Encapsulins are a class of BMCs characterised by their conserved subunit (Enc), which self-assembles to encapsulate enzymatically active cargoes and can remain porous to cargo substrates. The overall structure of Enc subunits across species with different T numbers is conserved and consists of a peripheral domain (P-domain), an axial domain (A-domain), and an extension loop (E-loop). T = 1 encapsulins of Mycobacterium tuberculosis, the causative agent of tuberculosis, and the closely related Mycobacterium marinum, are known to encapsulate the DyP as a core cargo with iron storage ferritin protein (BfrB)28 and FolB as possible secondary cargoes. In vitro cryo-electron microscopy (EM) single-particle analysis of the Mycobacterium tuberculosis encapsulin was used to obtain three structures of the encapsulin shell in intermediate states, as well as a 2.3 Å structure of the fully assembled shell.

In addition, we studied partial encapsulin structures to characterise stable encapsulin shell intermediates in vitro, by using low pH conditions to disassemble encapsulin shells, followed by reassembly at neutral pH. To explore the structural landscape of encapsulin shell formation, we used 2D and 3D (focused) classification and local symmetry to determine the structure of different stable encapsulin intermediates in an incomplete assembly state. This resulted in structures of three distinct intermediates of the encapsulin shell; a 48-mer (3,427 particles, 5.4 Å), a 52-mer (4,378 particles, 4.5 Å) and a 54-mer (6,294 particles, 4.6 Å). All three intermediates have an even number of monomers, appear to be closed on one side of the shell, and miss subunits on the other end. All three stable intermediates have an overall icosahedral structure with RMSD values for the 48,52 and 54-mer compared to the structure of the full shell of 1.08 Å, 0.60 Å and 2.66 Å respectively, although the 54-mer is, compared to the full encapsulin, flattened in one direction and elongated perpendicularly to it. The 52-mer consists of 39 fully resolved, and 13 less well resolved monomers, and the 54-mer consists of 27 fully resolved monomers and 27 less well resolved monomers. Not surprisingly, we observed higher cross-correlation values for Enctb monomers on the far side of the opening and lower cross-correlation values closer to the opening; in particular directly on the edges. On the edges of the intermediate encapsulin shells, we observed many points of three and fivefold symmetry with one or more Enctb subunits missing. However, all dimers (in total 77) have both Enctb subunits present, and where a subunit around five or three fold symmetry is missing, its dimeric partner is also missing. Our intermediate structures indicate that the structure of larger partial shells is largely icosahedral, with some deviations observed in the 54-mer.

>[54x]MNNLYRDLAPVTEAAWAEIELEAARTFKRHIAGRRVVDVSDPGGPVTAAVSTGRLIDVKAPTNGVIAHLRASKPLVRLRVPFTLSRNEIDDVERGSKDSDWEPVKEAAKKLAFVEDRTIFEGYSAASIEGIRSASSNPALTLPEDPREIPDVISQALSELRLAGVDGPYSVLLSADVYTKVSETSDHGYPIREHLNRLVDGDIIWAPAIDGAFVLTTRGGDFDLQLGTDVAIGYASHDTDTVRLYLQETLTFLCYTAEASVALSH Nalpha-[(benzyloxy)carbonyl]-N-[(1S)-3-chloro-1-methyl-2-oxopropyl]-L-phenylalaninamide 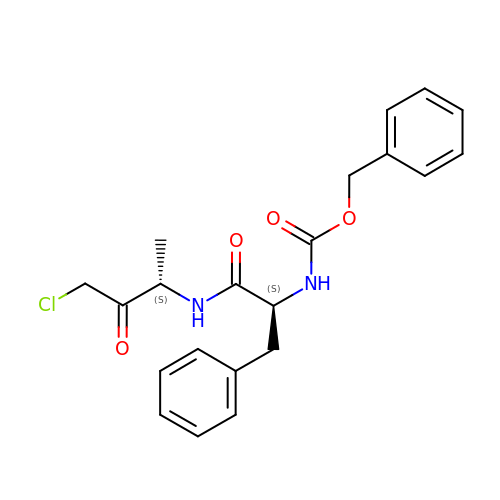| C21 H23 Cl N2 O4 | YAWCSFNDFRSZKD-YJBOKZPZSA-N> MWNPIVNVDITLNTAGTTREGFGLPLFLASTDNFEERIRGYTSLTEVAEDFDESTAAYKAAKQ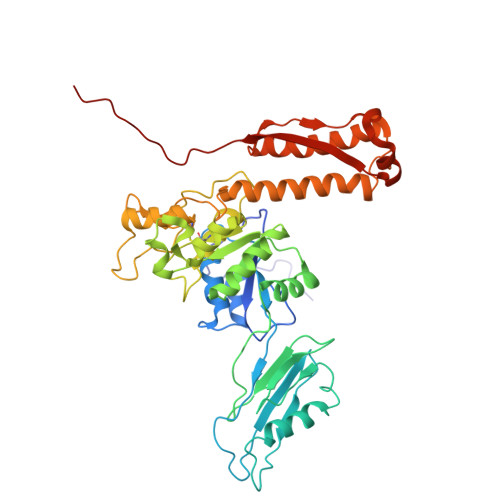LWSQTPKVTQLYIGRRTMQYTVSIPDTVAEGSEYSLTVAIGGGVSQPFQYTAKENDTALIVLNEFKSQIEASPTIKDGVNASVTGTGASATMIITKAGDNDFVKVTSITPTTSIAATTADTASAALASIETYSTDWYFISAEDRTQQFVLAMASEIQARKKIFFTANADVKALQGTDLTSATDVPAQLAKSKYTRTVCLWHHTAEFDYPEMAYIAYGAPYDAGSIAWGNAQLTGVAASLQPANQRPLISIQKSALDTRSCNFIDLDGGVPVVRRGITSGGEWIDIVRGVDWLESDLKTSLRDLLINQKGGKITYDDTGITRIRQVIETSLQRAVNRKFLSTYTVTVPKASQVALADKKARILKDITFHGILAGAILDVDLKGTVAYE>GVALGATRVIYPAGQKQEQLAVTNNDENSTYLIQSWVENADGVKDGRFIVTPPLFAMKGKKENTLRILDATNNQLPQDRESLFWMNVKAIPSMDKSKLTENTLQLAIISRIKLYYRPAKLALPPDQAAEKLRFRRSANSLTLINPTPYYLTVTELNAGTRVLENALVPPMGESTVKLPSDAGSNITYRTINDYGALTPKMTGVMEHHHHHH[4x];>[4x]HHHHHHGEVVNAACAVDAGSVDQTVQLGQVRTASLAQEGATSSAVGFNIQLNDCDTNVASKAAVAFLGTAIDAGHTNVLALQSSAAGSATNVGVQILDRTGAALTLDGATFSSETTLNNG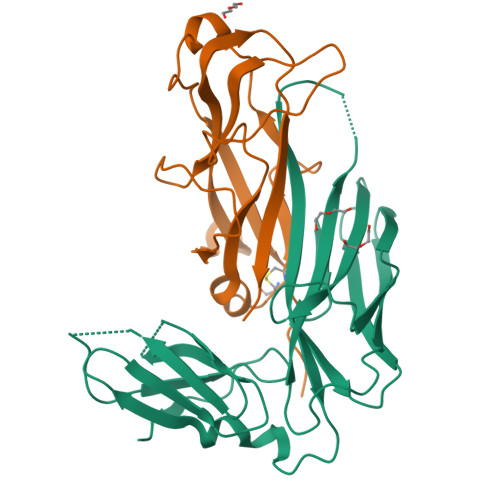TNTIPFQARYFATGAATPGAANADATFKVQYQ> NIPLEELQRNLQFHAFISYSGHDSFWVKNELLPNLEKEGMQICLHERNFVPGKSIVENIITCIEKSYKSIFVLSPNFVQSEWCHYELYFAHHNLFHEGSNSLILILLEPIPQYSIPSSYHKLKSLMARRTYLEWPKEKSKRGLFWANLRAAINIKL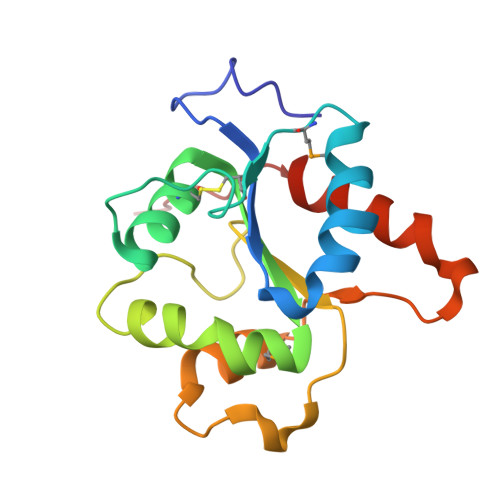TEQAK>[2x]MNKVHVSAVGTSLLKNSLSADNVKKEVEDLGLKDWDRLKFDDDRQNKIRDNFTTLKDLLLNFLKSKGKEASAELDSLLSAIEKLQHKKEELYVFLYTTNTWNSKLAGEVIKNYLEEEGIKSELATVKSISSEETFHEGIEDLFD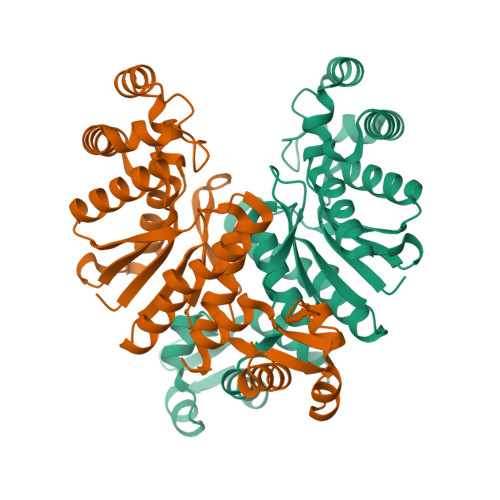KVIYKILKFKEEGKEVYINATAGLKPETTFLTLAGLLAGADLVYYKYQEFNDVVFLPSPPITISPRYLEWLIEFANYGYTLSEKKAEELGIPVRLLEVRNLVERKGEDAYRLKDWVRKMLGIYLGSEFELE>SNAIRPTIGQQMETGDQRFGDLVFRQLAPNVWQHTSYLDMPGFGAVASNGLIVRDGGRVLVVDTAWTDDQTAQILNWIKQEINLPVALAVVTHAHQDKMGGMDALHAAGIATYANALSNQLAPQEGMVAAQHSLTFAANGWVEPATAPNFGPLKVFYPGPGHTSDNITVGIDGTDIAFGGCLIKDSKAKSLGNLGDADTEHYAASARAFGAAFPKASMIVMSHSAPDSRAAITHTARMADKL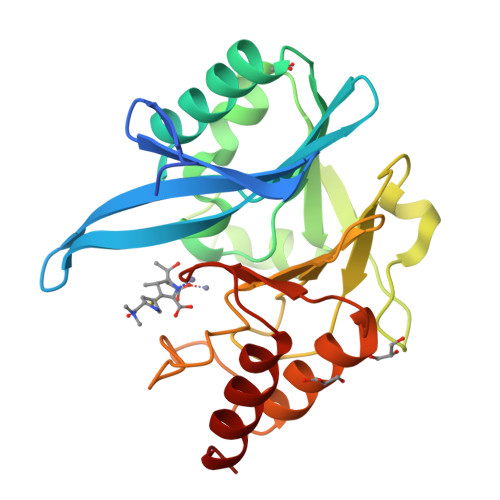R[2x]6-amino-3-{2-deoxy-5-O-[(R)-hydroxy{[(S)-hydroxy(phosphonooxy)phosphoryl]oxy}phosphoryl]-beta-D-erythro-pentofuranosyl}-3,4-dihydro-1,3,5-triazin-2(1H)-one 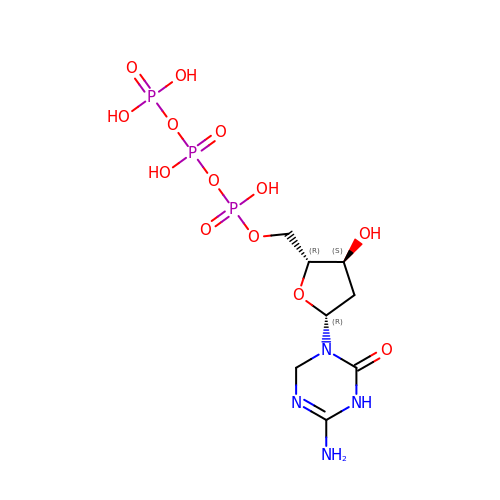| C8 H17 N4 O13 P3 | YEGZZVDXUFGWTE-KVQBGUIXSA-N>GSHMAGAQDFVPHTADLAELAAAAGECRGCGLYRDATQAVFGAGGRSARIMMIGEQPGDKEDLAGLPFVGPAGRLLDRALEAADIDRDALYVTNAVKHFKFTRAAGGKRRIHKTPSRTEVVACRPWLIAEMTSVEPDVVVLLGATAAKALLGNDFRVTQ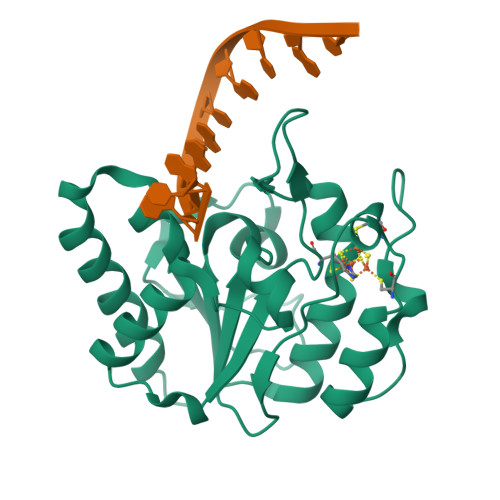HRGEVLHVDDVPGDPALVATVHPSSLLRGPKEERESAFAGLVDDLRVAADVRP[2x]S-Adenosyl-l-homocysteine hydrolase (SAHH) reversibly cleaves S-adenosyl-l-homocysteine, the product of S-adenosyl-l-methionine-dependent methylation reactions. The conversion of S-adenosyl-l-homocysteine into adenosine and l-homocysteine plays an important role in the regulation of the methyl cycle. SAHH depends on the cofactor nicotinamide adenine dinucleotide in its oxidised form (NAD+), which is self-regenerated during the catalytic cycle. The protein structure of SAHHs features three domains in a monomer, the active form is usually a homotetramer19.

Structures of archaeal SAHHs were determined from three organisms: Methanococcus maripaludis (MmaSAHH), Pyrococcus furiosus (PfuSAHH), and Sulfolobus acidocaldarius (SacSAHH). While archaeal enzymes deriving from the Crenarchaeota phylum (SacSAHH and SsoSAHH) show catalytic activity only with SAH, homologues from T. maritima and the euryarchaeal classes of Methanococci and Thermococci (MiSAHH, MjSIHH, PfuSAHH, TkSAHH, and MmaSAHH) show higher catalytic activity with SIH. Regarding the structures of PfuSAHH and MmaSAHH with their preferred substrates inosine or SIH, the oxygen attached to C6 seems to form additional hydrogen bonds with the carbonyl oxygen atoms of Asp348 (PfuSAHH) or Asp362 (MmaSAHH) in the main chains. This suggests that the hypoxanthine ring is in the imino-hydroxy form, although inosine has been shown to be most stable in the amino-oxo form in water. Similarly, our complexes of PfuSAHH and MmaSAHH with inosine and the complex of SacSAHH with adenosine show a closed conformation state of the molecular gate in their active site. The absence of a comparable monovalent cation was observed in all structures of archaeal enzymes. Similarly, MmaSAHH tetramers and SacSAHH tetramers exhibited an average ΔGint value of −133.5 kcal mol−1 and −127.5 kcal mol−1, respectively.

>MGSSHHHHHHSSGLVPRGSHMSNVKDMSLAPSGHLKMEWAKRHMPVLCRIAEEFKNDKPFEGLTIGMALHLEAKTAILAETLLEGGAKIVITGCNPLSTQDDVAAACVEKGMEVYAWRGETNEEYYENLNKVLDSNPDIIIDDGADLIFLIHTERTELIGKIMGGCEETTTGIIRLKSMAEEGALKFPVVNVNDAYTKHLFDNRYGTGQSAMDGIIRTTNLLIAGKNVVVGGYGWCGRGVASRAAGHGANVIITEVNPIRALEAKMDGFTVLKMEEAAKIGDIFVTTTGCKDILRMEHFLLMKDGAVLSNAGHFDNEINKNDLKELSKSVKEARFNIEEYDLGNKKIYLLGEGRLVNLACADGHPCEVMDMSFANQALSAKFIKENKGKLENEVYEIPYEQDFKIALLKLHSMGADIDELSPEQRKYLSDWKEGT[8x]>ALSTEVVHLRQRTEELLRCNEQQAAELETCKEQLFQSNMERKELHNTVMDLRGNIRVFCRIRPPLESEENRMCCTWTYHDESTVELQSIDAQAKSKMGQQIFSFDQVFHPLSSQSDIFEMVSPLIQSALDGYNICIFAYGQTGSGKTYTMDGVPESVGVIPRTVDLLFDSIRGYRNLGWEYEIKATFLEIYNEVLYDLLSNEQKDMEIRMAKNNKNDIYVSNITEETVLDPNHLRHLMHTAKMNRATASTAGNERSSRSHAVTKLELIGRHAEKQEIS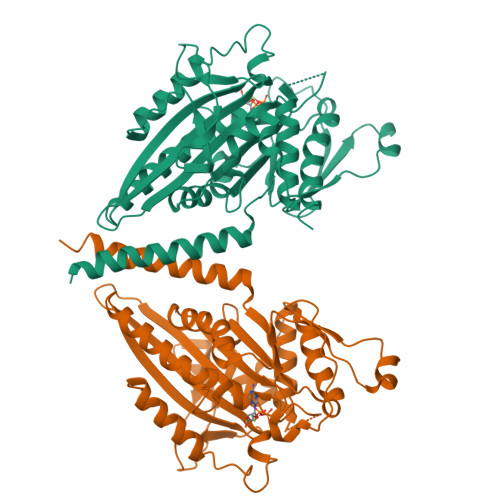VGSINLVDLAGSESPKTSTRMTETKNINRSLSELTNVILALLQKQDHIPYRNSKLTHLLMPSLGGNSKTLMFINVSPFQDCFQESVKSLRFAASVNSCKMTKAKRNRYLNNSVANSSTQSNNSGSFDK[4x]As such, we found that a circularly permuted variant of a cage-forming enzyme, Aquifex aeolicus lumazine synthase, cpAaLS, assembles into a variety of hollow spherical and cylindrical structures in response to changes in ionic strength. Cryogenic electron microscopy revealed that these structures are composed entirely of pentameric subunits, and the dramatic cage-to-tube transformation is attributed to the moderately hindered 3-fold symmetry interaction and the imparted torsion angle of the building blocks, where both mechanisms are mediated by an α-helix domain that is untethered from the native position by circular permutation. While the wild-type protein, AaLS-wt, self-assembles into a ∼ 16 nm dodecahedral structure composed of 60 identical monomers,35 the negatively supercharged variants AaLS-neg and AaLS-13 adopt expanded 360- and 720-mer assemblies, respectively, constructed entirely from pentameric capsomers. Moreover, a circularly permuted variant of AaLS, cpAaLS(119), forms not only ∼24 nm and ∼28 nm expanded spherical cages, but also straight ∼24 nm-wide tubes of variable length. We previously designed two circularly permuted variants of AaLS and confirmed that their morphologies depend on the positions of the newly generated N- and C-termini. The native terminal amino acids were connected via an octapeptide linker using genetic fusion and new sequence termini were introduced either between residues 84 and 85 or 119 and 120, yielding cpAaLS(84) or cpAaLS(119), respectively.

Further increasing NaCl concentration to 0.35 M yielded a mixture of the tubes and ∼28 nm spherical cages ∼44% and ∼46%, respectively. The 24 and 28 nm spherical cages are composed of 24- and 36-pentamers, respectively, and both have tetrahedral symmetry, resembling those formed by the previously engineered AaLS variants, NC-1 and AaLS-neg. In contrast, cpAaLS(119) assemblies are non-quasi-equivalent, where at least one interface of the pentameric subunits remains uncontacted. While the number of pentamer–pentamer contacts remains 0 or 1 without NaCl at pH 8.5, judged by the 2D-averaged cryo-EM images, the mean contact number per pentamer increases to 3, 3.7, and 4 in the tubular, 28 nm-, and 24 nm spherical cages, respectively. The bonding network observed at the 2-fold symmetry interface of AaLS-wt is approximately preserved for all the interacting pentamers in the cpAaLS(119) assemblies. In marked contrast, the (pseudo) 3-fold symmetrical interaction interface of cpAaLS(119) assemblies lacks cryoEM density corresponding to the N-terminal α-helix(120–131). This finding suggests that the α-helix is unable to form the native-like hydrophobic cluster, likely due to the disconnection of residues 119 and 120 for circular permutation. The α-helix(120–131) domain is structurally disordered and unseen in cryo-EM analysis of the cpAaLS(119) spherical cages.

>[180x]MTLEQAIERAGTKHGNKGWEAALSAIEMANLFKSLRGTGGSGSSMEIYEGKLTAEGLRFGIVASRFNHALVDRLVEGAIDCIVRHGGREEDITLVRVPGSWEIPVAAGELARKEDIDAVIAIGVLIRGATPHFDYIASEVSKGLANLSLELRKPITFGVITAD> MDGSRGTAPGGDDLRGDRRDSYQGEDREDSHLLGALEDGNHQQSQGHGGGSGFYHHNVNSSSASVLEGVEMAHDELFAGPVAESVPTSVSAFSHRHGRAESVASFSFYHEQDDQREELEAPPGSLGARLSIDDLDELPFEEEGLSESEMPEQLDTFGIDLEWGSMNNGYPLIRRSSTHSQFSAHHRLLRRESGVSAASGYTGGRSSQKMRLDNDDLTIAISGFITNRIGFAIYIVLCVLTGGIAWLFLRWYPKYYVKLVGCATPFRDCQWVVIEDHFNKMTILSIRVKPYNRPLSTVFGTPSRATSWPLAQDPDPVLRELRSITYCYYKFYYHPVLDKFFCCNGWKDPQWNSMQNARSGLHGDEKAHREAVFGPNSIDVDEQSILQLLVSEILTPFYAFQVFSLILWLCDEYYYYAAAILLISAGSIITSLLETKETRRRLREMSRFECEVRVFRGGFWRTFPSSDLVPGDVYEVSDPSLTQIPADSLLLTGDCIVNESMLTGESVAVSKTPATNETLAKLNPAASTFSHDVDKHFLYCGTKLIRARQRLADTDEAAAVALVVRTGFNTTRGALVRSMLVPKPSKFKFYEDSFRYLKVMGCLAGLAFIVSLVNFIRLKLHWTLILLRALDLLTIVVPPALPATLTIGTSFAVQRLKGKKIFCTSPQRVNVGGKIDLMCFDKTGTLTEEGLDVLGIRVASRVSNRFTELLTNVDDLTWSCDSVSNGDEVKPADHVDGSSLKKDKTKPLDPYRAALYVMASCHSLRIVDGVAVGDPLEVKMFEFTGWSYEEGFIAGEVISTEGRGDISPSIARPPRYMTSQEMSIGEAPPAVGVLRAFDFNPLLRRSSVIARVVGNSGGYALVKGSPECMPEIC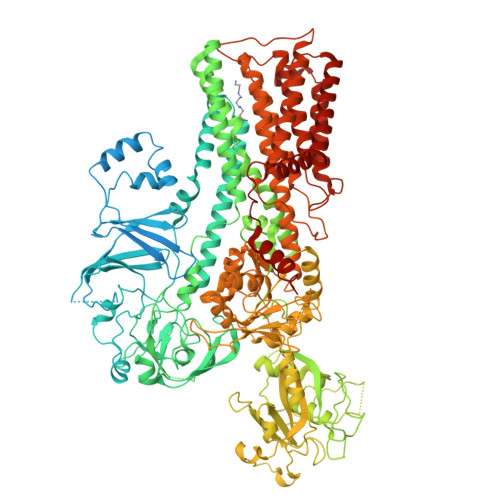RPETLPSDFDELLSYYTHAGYRVIACATKRIPKLNLVSVNRMTRDEVESGLDFVGFIIFENKLKPTTTSVIKELLSSNIGTVMITGDNIRTAVSVARQCGIIEEHAHCYMPRFIEGNADDCNAKLRWESINNPALELDPWTLLPMPVPPQTDASLPYDVSNIRNYAIAVTGDVFRWIVDHAPTDVLHRMLVLGKVYARMSPDEKQELVKKFQSIDYSCGFCGDGANDCAALKAADVGISLSEAEASVAAPFTSQIFDIRCVPEVIREGRASLVTSFSCFKYMSLYSFIQFTSVSFLYVSASNLGDFQFLYIDLMLILPIAVFMSWAGPHSKLCAKRPVSDLVSRKVLVPLLSHVFVCVMIQALAWVAVRQQPWYIPPIVDTEKSNIENSENTTLFFASCFEYILSGVVLNAGRPFRQSPLETWPFLSAVAVTLIATLLMLLVPPYWLFEFMQLTWMSWTFKITLIAFGFVYFLIAWTGEHYLFLWLARFLGRMRQRLFKQPKQRKLYKIVKEKLVFENLYFQ16,17-dimethoxy-21-(2-pyridin-4-ylethyl)-5,7-dioxa-13$l^{4}-azapentacyclo[11.8.0.0^{2,10}.0^{4,8}.0^{15,20}]henicosa-1(13),2,4(8),9,14,16,18,20-octaene 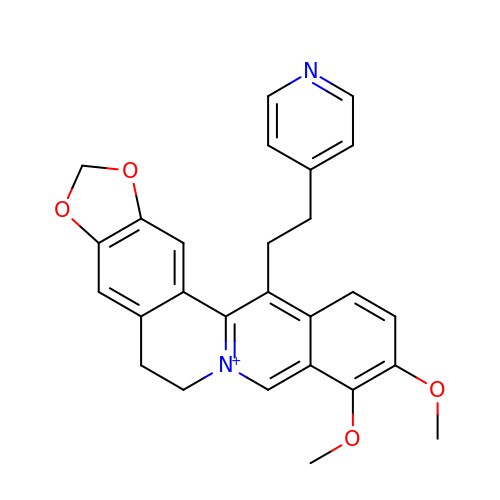| C27 H25 N2 O4 | RNEIDRUOMNDERD-UHFFFAOYSA-N>SGAMYIDCDGIKLNAYLDMPKNNPEKCPLCIIIHGFTGHSEERHIVAVQETLNEIGVATLRADMYGHG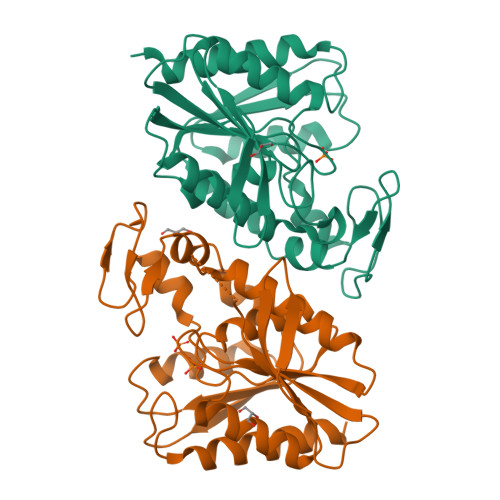KSDGKFEDHTLFKWLTNILAVVDYAKKLDFVTDIYMAGHSQGGLSVMLAAAMERDIIKALIPLSPAAMIPEIARTGELLGLKFDPENIPDELDAWDGRKLKGNYVRVAQTIRVEDFVDKYTKPVLIVHGDQDEAVPYEASVAFSKQYKNCKLVTIPGDTHCYDHHLELVTEAVKEFMLEQIAK[4x]>[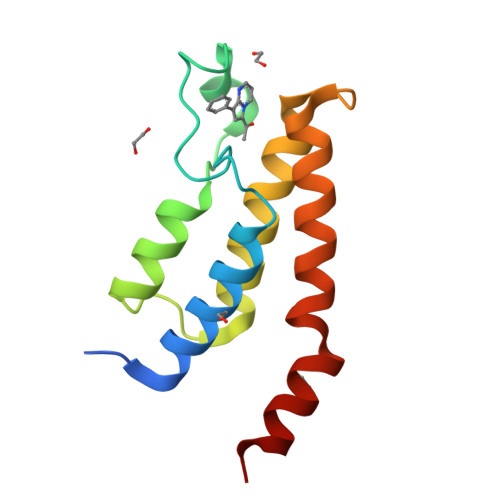2x]LKLSAENESTPIQQLLEHFLRQLQRKDPHGFFAFPVTDAIAPGYSMIIKHPMDFGTMKDKIVANEYKSVTEFKADFKLMCDNAMTYNRPDTVYYKLAKKILHAGFKMMSKERLLALKRSMS> PHTN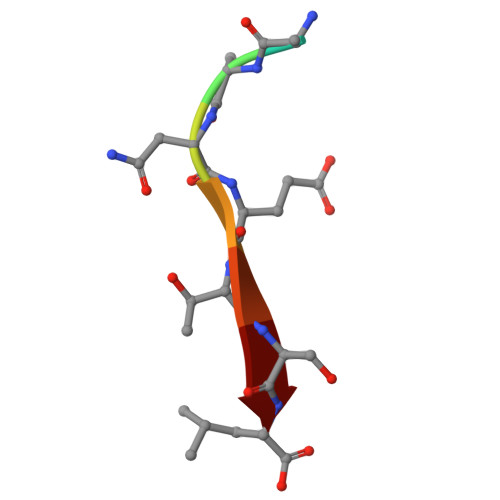ETSL>PVMHPHGAPPNHRPWQMKDLQAIKQEVSQAAPGSPQFMQTIRLAVQQFDPTAKDLQDLLQYL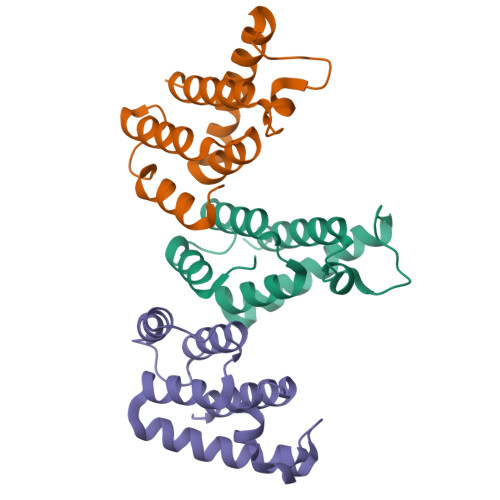CSSLVASLHHQQLDSLISEAETRGITGYNPLAGPLRVQANNPQQQGLRREYQQLWLAAFAALP[3x]>[5x]VRTCLPCGPGGKGRCFGPSICCGDELGCFVGTAEALRCQEENYLPS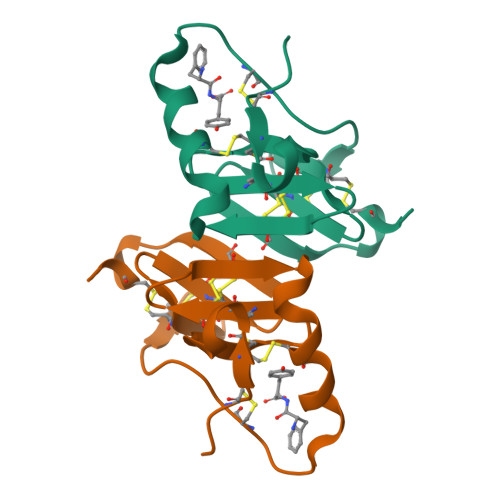PCQSGQKPCGSGGRCAAAGICCSPDGCHEDPACDP>[2x]TKIAMANFKSAMPIFKSHAYLKELEKTLKPQHFDRVFVFPDFFGLLPNSFLHFTLGVQNAYPRDCGAFTGEITSKHLEELKI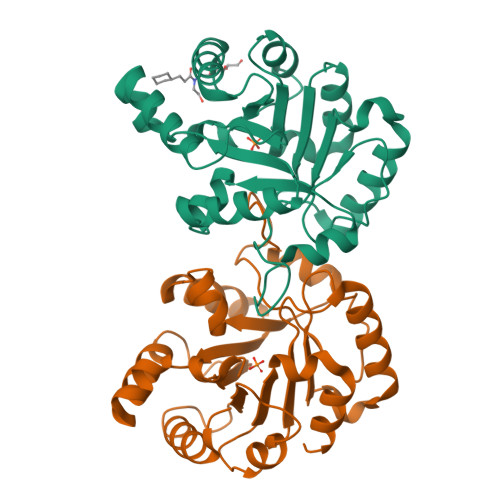HTLLIGHSERRTLLKESPSFLKEKFDFFKSKNFKIVYCIGEELTTREKGFKAVKEFLSEQLENIDLNYPNLVVAYEPIWAIGTKKSASLEDIYLTHGFLKQILNQKTPLLYGGSVNTQNAKEILGIDSVDGLLIGSASWELENFKTIISFL>[2x]VTPPPEKFNFAEHLLQTNRVRPDKTAFVDDISSLSFAQLEAQTRQLAAALRAIGVKREERVLLLMLDGTDWPVAFLGAIYAGIVPVAVNTLLTADDYAYMLEHSRAQAVLVSGALHPVLKAALTKSDHEVQRVIVSRPAAPLEPGEVDFAEFVGAHAPLEKPAATQA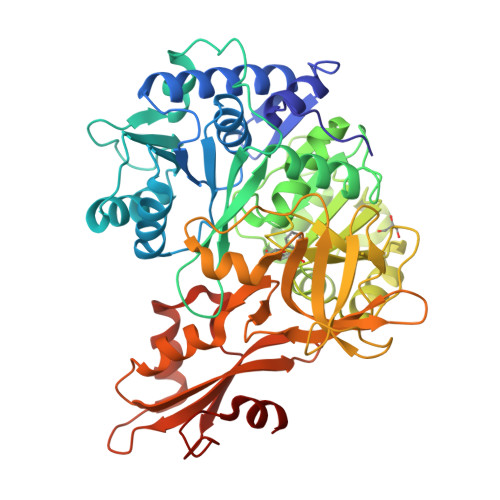DDPAFWLYSSGSTGRPKGVVHTHANPYWTSELYGRNTLHLREDDVCFSAAKLFFAYGLGNALTFPMTVGATTLLMGERPTPDAVFKRWLGGVGGVKPTVFYGAPTGYAGMLAAPNLPSRDQVALRLASSAGEALPAEIGQRFQRHFGLDIVDGIGSTEMLHIFLSNLPDRVRYGTTGWPVPGYQIELRGDGGGPVADGEPGDLYIHGPSSATMYWGNRAKSRDTFQGGWTKSGDKYVRNDDGSYTYAGRTDDMLKVSGIYVSPFEIEATLVQHPGVLEAAVVGVADEHGLTKPKAYVVPRPGQTLSETELKTFIKDRLAPYKYPRSTVFVAELPKTATGKIQRFKLREGVLG>MSLKPDNLPVTFGKNDVEIIARETLYRGFSSLDLYRFRHRLFNGQMSHEVRREIFERGHAAVLLPFDPVRDEVVLIEQIRIAAYDTSETPWLLEMVAGMIEEGESV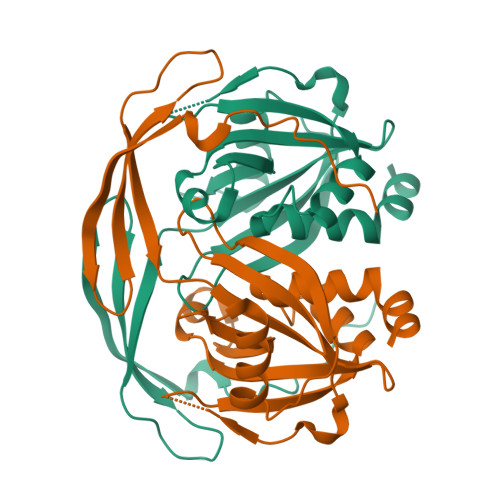EDVARREAIEEAGLIVKRTKPVLSFLASPGGTSERSSIMVGEVDATTASGIHGLADENEDIRVHVVSREQAYQWVEEGKIDNAASVIALQWLQLHHQALKNEWAEGGSHHHHHH[3x]> GSSSGGSGHTPTTQATHADDHDLTTHNGTEEHDDGHDDGHDDLHAHAPKVIVFISGSCLFGAISRSLFKKLPIPYTVVLLILGAILGVVASNVPLVEEHTRDVAHMDPHVLLQIFLPVLIFESAFAMDVHTFMRSFSQVCILALFGLVVASVLTAVLAMNLFNYNWNFSEAMMFGAIMSATDPVAVVALLKDLGASKQLGTIIEGESLLNDGCAIVIFNVFMKMVFFPQLTSTVGQNVLYFLQVAVAGPLWGYAVAKVTVFFLSHIFNDALVEITITLAATYLTYYIGDIWLEVSGVLAVVVLGLIVNAEKTSISPEVEVFLHRFWEMLAYLANTLIFMMVGVVVTQKALVAVDKMDWFYLIILYLAITIIRGMVISLFSPILSRIGYGLTWRNAVIMTWGGLRGAVGLALALVVENLAGNDVIGSKFLFHTAGIVVLTL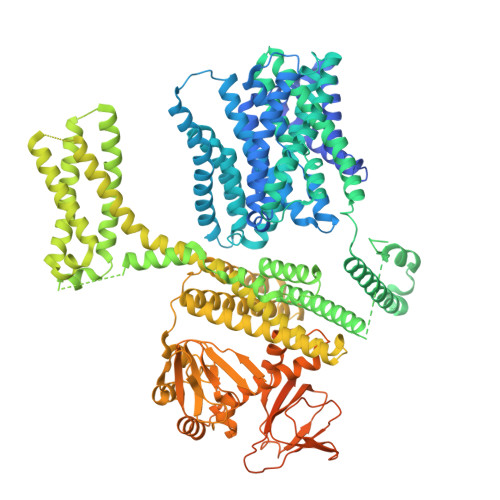VINATTIQTLLRILGMSDISIPKRLAMAGAVRRIHEGQNRTLNMLKSDRFLADADWDIATAACEISDPYSALSDDENAPADELTLGERKSVCPGCKAMVPNEPSPREFADMMEEARLRMLKAEKISYWKQFEHGMLAREALRLLVQHAEVAADEKDQFILVDDLKKSWQIKGIYPWLKRKLEDLISEKKIAAIPMPKYKLGKLMYKICHHMAFEVTINIAIVLNIVPIIMEFVVQDKMASVSTMAAPGSTVSSEPSSLQKIEDALRISNYVFFVIYAIEAIVKILGLGRHYIVSHWNKFDAFILVVALVDIIIAETLLKGSITINLSSIKVVKLFRLLRGLRMLRLTKALIPKLILVVNGKINNQLSLGYDVGKGYIIGEEEVGKIIDRMVDNKKILRELKHISETGRLQVVKELGLLQREHPGIAVSVKTRQAIRTILNHSRETIHELQGAGLLDEMEAHKLELTVEIKMKRLMNAPSSIPPPPPENLLKNVSWLAGDMKLIDFIKARASLLHFDYGEVIVREGDESDGLFLIVSGLVKLYGKSAFLDHDNPPVTAGSEENEVFEDYLTVGNVIGEMGVLTKKPRNATVTCETTVQVYFITAEDMNIAIDTFTLYPSLEYRLWRVVAIRIATPLIMEQMAFQGWTQEKVKLHLERGYLVDLAESHFQFNIDATLEDVILINGTAYNAHTREEIRSPCLISRTVHKLTFQYTATEEPRLFVVRNAEYNGPILDGRLDVDSKRSLISITEISSNMCLKHAAELRQKNSKVMLSRKSSGAAAKEEEDCIPNTSDVEQAAGVSPSVPTKTTPKPKSFLPSLGLSMSKERVNGEAVEESPVKTKQGEETPETEEGAAPRVNVASNSLEVLFQ> MEIVIRTGSGDVRGSKENGIAVFRGIPYAEPPVGAHRFTAPRPPRPWDGVRDATEFSATAPRPPYPEAIGALLIERFIPGDDYLTLNVWTPDPNAVGLPVMVWIHGGAFTNGSGSEPVYDGAAFARDGVVFVSFNYRLGIIGFADLPDAPSNRGLLDQIAALEWVRDNIARFGGDPGNVTVFGESAGAMSVCTLMATPRARGLFRRAILQSGAGNMAVAAEDATTIAAVIAHRLGVEPTAAALAHVPVAQLLDVQQQVAQEIQGAPDPAVWGERIAGGSVLLPFAPVIDGELLSQRPAEAIAGGAGHDVDLLFGTTTDEYRLFLAPTGLLPFITSDYVTAHLAKSGLDADAAKAYTAEGRGEEPGDILASIITDQVFRIPALRIAESRVDAPARTFGYEFAWRTPQLDGILGACHAVELPFVFRTLDRAASLVGTNPPEELAETVHN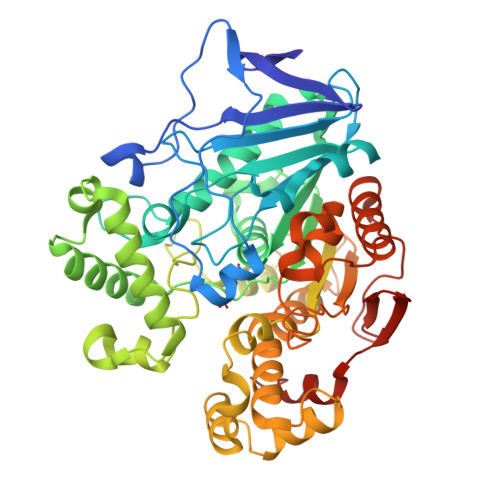AWVRFATSGDPGWPAWNPETRSVMRFDHPVSEMVTDPYPATRALWDGVPL> MRNKIFISHATPDDNDFTRWLALKLIGLGYEVWCDILFLDKGVDFWSNIEKVIREDTCKFLLVSSSYSNQREGVLKELAVAAKVKKQLKDDKFIIPLAIDEQLSYDDINIDIVRLNAIDFKMSWARGLKDILEAFEKQKVPKEVADASKSNLLYQQIFLHDKSVIEKEEIYDSNWLSILSFPEELRFHEYNWMLPKRFDVRELTFPAVRYKNYLCTFAW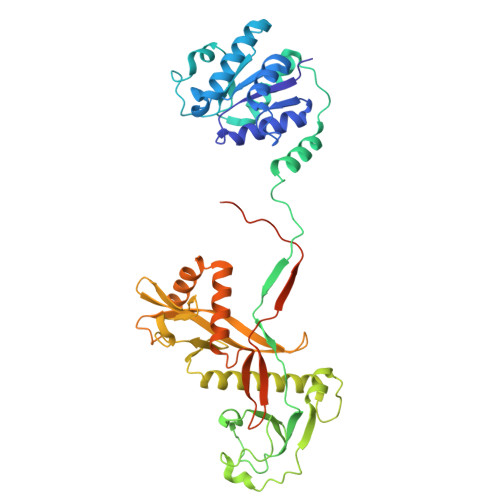AYDFTYHLPKTETYHKSKTIRIPTEEILSGSYDSNFIRNAECKRLIVQLLNKAFELRMKDKEVQEYEMSNKTAYWLEKGKLEKDKFEKTMLVGKQKDKNWHFAISGASKLYPFPVLMISSHIFFTADGKKLIDSSSVQHSSRRRQGKNWWNNTWRTKLLAFIKYLSDDDTSFYLEMGSEEKVFVSNEPVKFKGNVSYNIPEKNTLEEEAELSGFNQGEDIEELEELIENLEAE> GSNMVKVPECRLADELGGLWENSRFTDCCLCVAGQEFQAHKAILAARSPVFSAMFEHEMEESKKNRVEINDVEPEVFKEMM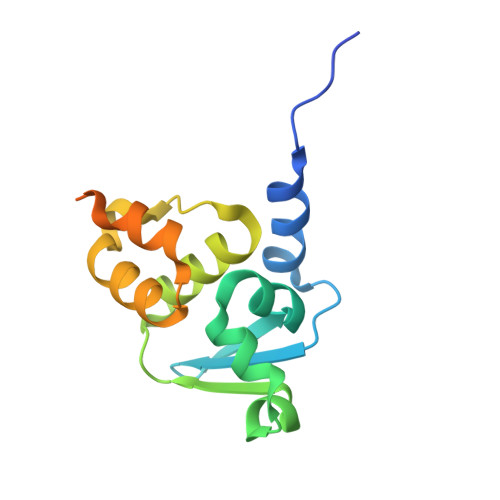CFIYTGKAPNLDKMADDLLAAADKYALERLKVMCEDALCSNLSVENAAEILILADLHSADQLKT> GSNHHRGLASANVDFAFSLYKHLVALSPKKNIFISPVSISMALAMLSLGTCGHTRAQLLQGLGFNLTERSETEIHQGFQHLHQLFAKSDTSLEMTMG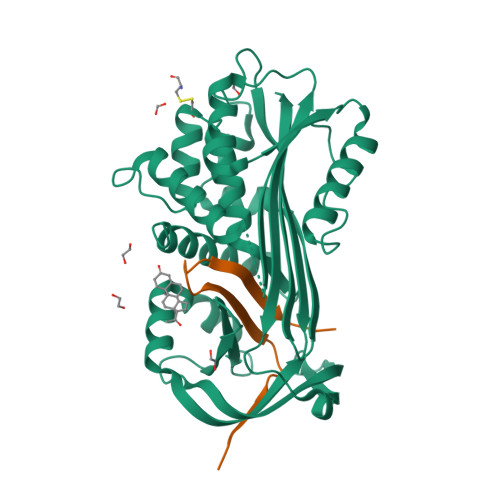NALFLDGSLELLESFSADIAHYYESEVLAMNFQDWATASRQINSYVKNKTQGKIVDLFSGLDSPAILVLVNYIFFKGTWTQPFDLASTREENFYVDETTVVKVPMMLQSSTISYLHDSELPCQLVQMNYVGNGTVFFILPDKGKMNTVIAALSRDTINRWSAGLTSSQVDLYIPKVTISGVYDLGDVLEEMGIADLFTNQANFSRITQDAQLKSSKVVHKAVLQLNEEGVDTAGSTGVTLNLT;> SKPIILRFNQPFIIMIFDHFTWSSLFLARVMNPV To gain insight into IniA-mediated drug resistance, we determined the structure of full-length IniA from Mycobacterium smegmatis (M. smegmatis), which shares 68% sequence identity with IniA from Mycobacterium tuberculosis (M. tuberculosis). IniA consists of an N-terminal GTPase domain and two HBs. Here, we determined structures of IniA, with and without bound GTP, and demonstrated that it mediates membrane fission in vitro. Our results suggested that IniA, like other BDLPs, has weak GTPase activity and nucleotide-dependent dimerization in solution, but tends to form nucleotide-independent homotypic interactions on the membrane and cuts the membrane.

IniA was expressed in E. coli, purified, and crystallized in the presence of GTP. A 2.2 Å resolution structure was determined by the single-wavelength anomalous diffraction (SAD) method. One IniA molecule is present in the asymmetric unit. Even though there is only a monomer present in the asymmetric unit of the GTP-bound IniA structure, through crystallographic symmetry a similar dimer is also observed in that complex. Four signature motifs wrap around GTP: G1 (P-loop), G2 (switch 1), G3 (switch 2), and G4. As expected, K49 and S50 in the G1, T70 in G2, and D141 in G3, with the help of a magnesium ion, coordinate the binding of the phosphate moieties in the nucleotide. K200 and D202 in G4 engage the ribose. K46 in G1, equivalent to the catalytic R77 of human atlastin 1 (ATL1, another dynamin-like GTPase that mediates fusion of the endoplasmic reticulum), points toward the bridging oxygen between the beta-phosphate and gamma-phosphate, suggesting a role in charge compensation during GTP hydrolysis. Furthermore, the G2 of IniA forms a U-shaped flap on top of GTP, likely stabilizing the positions of several key residues in the catalytic core. Analyzing the lipid-binding mode, we found a tartaric acid (TA) molecule (from the crystallization buffer) bound next to the predicted TM region.

> MGVIVELIDHTSAIAAAKDRADLVERLRAAKARISDPQIRVVIAGQLKQGKSQLLNSLLNIPVARVGDDESTVLATVVSYGEQASARLVVARPDGAEPELIEIPPSEVTTDLRRAPQASGRQVLRVEVTAPSPLLKGGLAFVDTPGVGGHGQPHLSATLGLLPDADAMLMISDTSQEFTEPEMKFIRQALEICPVAAIVATKTDLYPHWRQIVDANIAHLQRAGLNVPVIPASSVLRSHAISLNDKELNEESNFPAIVKFLSEHVLSRQNDRIRDQIVDEIRSAAEHLLLAVESELSSFNDPGERERLTAELERRKQEAQDALQQTALWQQVLSDGIADLTADVDHDLRHRFRIIAAHTEKVIDGCDPTLHWAEIGAELEDAVATAVGDNFVWAYQRAEALAAEVARTFTEAGLDAVQMPQIDARDMGAGFGELNSLARLEAKPIKIGHKVVTGMRGSYGGVLMFGMLTSFAGLGMFNPLSLGAGFVLGRKAYKEDMENRMLRVRNEAKANVRKFVDDVAFVVGKESRDRLKGIQRQLRDHYREIANQTTRSLNESLQAAIAAAKVEEAERNTRVKELERQQNILKQVVDHAAKLAAALEHHHHHH> MASAAVANYEEEIVRPVADFSP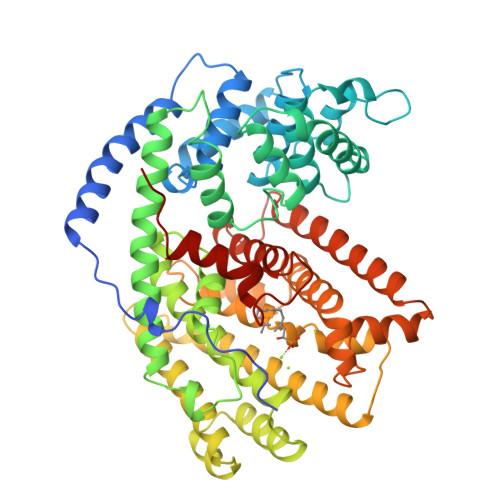SLWGDQFLSFSIDNQVAEKYAQEIEALKEQTRSMLLATGRKLADTLNLIDIIERLGISYHFEKEIDEILDQIYNQNSNCNDLCTSALQFRLLRQHGFNISPEIFSKFQDENGKFKESLASDVLGLLNLYEASHVRTHADDILEDALAFSTIHLESAAPHLKSPLREQVTHALEQCLHKGVPRVETRFFISSIYDKEQSKNNVLLRFAKLDFNLLQMLHKQELAQVSRWWKDLDFVTTLPYARDRVVECYFWALGVYFEPQYSQARVMLVKTISMISIVDDTFDAYGTVKELEAYTDAIQRWDINEIDRLPDYMKISYKAILDLYKDYEKELSSAGRSHIVCHAIERMKEVVRNYNVESTWFIEGYTPPVSEYLSNALATTTYYYLATTSYLGMKSATEQDFEWLSKNPKILEASVIICRVIDDTATYEVEKSRGQIATGIECCMRDYGISTKEAMAKFQNMAETAWKDINEGLLRPTPVSTEFLTPILNLARIVEVTYIHNLDGYTHPEEVLKPHIINLLVDSIKI>GPLGSMEPEEYRERGREMVDYICQYLSTVRERRVTPDVQPGYLRAQLPESAPEDPDSWDSIFGDIERIIMPGVVHWQSPHMHAYYPALTSWPSLLGDMLADAINCLGFTWASSPACTELEMNVMDWLAKMLGLPEHFLHHHPSSQGGGVLQSTVSESTLIALLAARKNKILEMKTSEPDADESSLNARLVAYASDQAHSSVEKAGLISLVKMKFLPVDDNFSLRGEALQKAIEEDKQRGLVPVFVCATLGTTGVCAFDCLSELGPICAREGLWLHIDAAYAGTAFLCPEFRGFLKGIEYA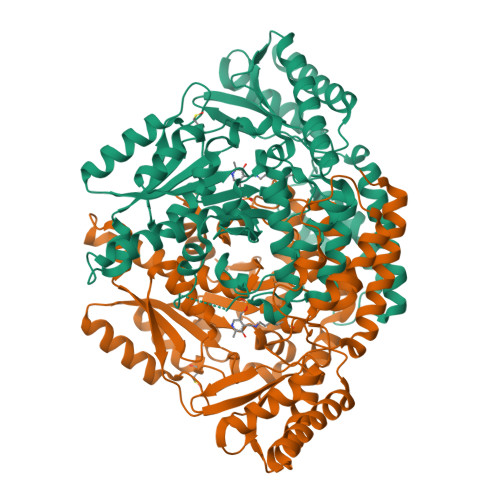DSFTFNPSKWMMVHFDCTGFWVKDKYKLQQTFSVNPIYLRHANSGVATDFMHWQIPLSRRFRSVKLWFVIRSFGVKNLQAHVRHGTEMAKYFESLVRNDPSFEIPAKRHLGLVVFRLKGPNSLTENVLKEIAKAGRLFLIPATIQDKLIIRFTVTSQFTTRDDILRDWNLIRDAATLILSQ[2x]> G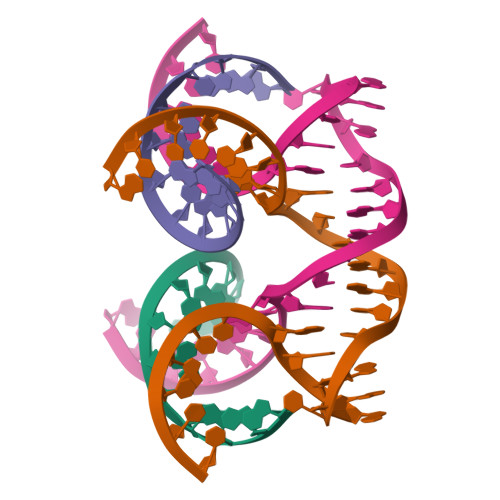GACAGAUGGGAG;> GCTCCCAGGCTAGCTACAACGACTGTCC> KEMSDRVLIFAVDASGSAAVARLSEAKGAVELLLGRAYAARDHVSLITFRGTAAQVLLQPSRSLTQTKRQLQGLPGGGGTPLASG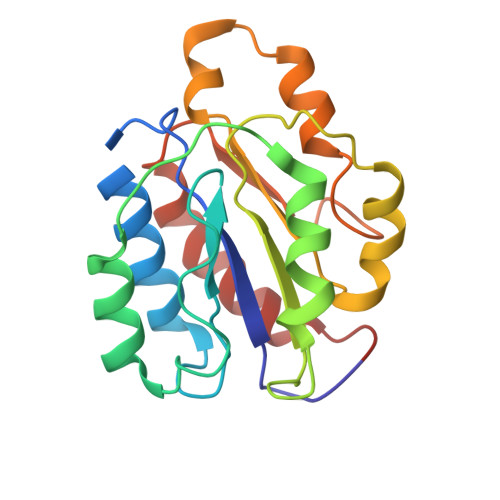MEMAMVTAKQARSRGMTPTIALLTDGRGNIALDGTANRELAGEQATKVARAIRASGMPAVIIDTAMRPNPALVDLARTMDAHYIALPRATAHKMADVLGAALEA>GAKTWVLTNAEEGIDKGNWQINSDQLKVKDHAFSIEQKVLHGGKQEGSKILTIHSKDGLTITLSPTRGMNLLRIEGFGSRMGWDSPVKEVVNPAFINLESRNGLGWLEGFNEMMVRCGYEWTGHPVTADGQIYTLHGKAGNTPASLVEVEVADSAPYEIRIRGLV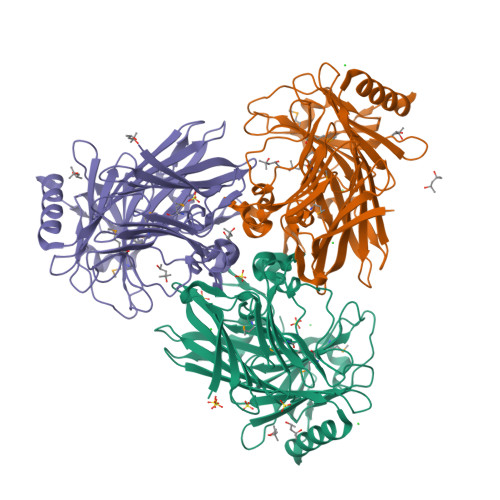KESTFKKADLQTLTELRYVPGSNSFSLHDVLTNHADYPHDYQIIYHSNFGTPILEEGARFLAPISSISPFNDYAKSGLKTWQTYQGPTKDFDEMVFNIQPLADENHQTLAAVVNKAGDKGASIQFDTRQLPVLTLWKNTDTVKQGYVTGIEPGTSYAYPVTIERKQKRVKQLQPGASAQFDLTYTLLHDSAQVAAVEQKIAKIQGDNKVAENETPIAKE[3x]> SMGFWEASSRGGGAFSGGEDASEGGAEEGAGGAGGSAGAGEGPVITALTPMTIPDVFPHLPLIAITRNPVFPRFIKIIEVKNKKLVELLRRKVRLAQPYVGVFLKRDDSNESDVVESLDEIYHTGTFAQIHEMQDLGDKLRMIVMGHRRVHISRQLEVEPEEPEAENKHKPRRKSKRGKKEAEDELSARHPAELAMEPTPELPAEVLMVEVENVVHEDFQVTEEVKALTAEIVKTIRDIIALNPLYRESVLQMMQAGQRVVDNPIYLSDMGAALTGAESHELQDVLEETNIPKRLYKALSLLKKEFELSKLQQRLG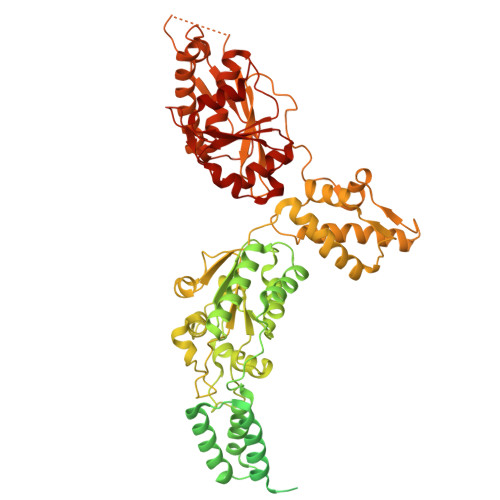REVEEKIKQTHRKYLLQEQLKIIKKELGLEKDDKDAIEEKFRERLKELVVPKHVMDVVDEELSKLGLLDNHSSEFNVTRNYLDWLTSIPWGKYSNENLDLARAQAVLEEDHYGMEDVKKRILEFIAVSQLRGSTQGKILCFYGPPGVGKTSIARSIARALNREYFRFSVGGMTDVAEIKGHRRTYVGAMPGKIIQCLKKTKTENPLILIDEVDKIGRGYQGDPSSALLELLDPEQNANFLDHYLDVPVDLSKVLFICTANVTDTIPEPLRDRMEMINVSGYVAQEKLAIAERYLVPQARALCGLDESKAKLSSDVLTLLIKQYCRESGVRNLQKQVEKVLRKSAYKIVSGEAESVEVTPENLQDFVGKPVFTVERMYDVTPPGVVMGLAWTAMGGSTLFVETSLRRPQDKDAKGDKDGSLEVTGQLGEVMKESARIAYTFARAFLMQHAPANDYLVTSHIHLHVPEGATPKDGPSAGCTIVTALLSLAMGRPVRQNLAMTGEVSLTGKILPVGGIKEKTIAAKRAGVTCIVLPAENKKDFYDLAAFITEGLEVHFVEHYREIFDIAFPD> MAEYFTYSKKRKEFNNPINFQDTETRYGGIQNQVVNINQYVQRNPNFIDLDNIAELSEHSVNTERVKTGDRGMSHKEGGWPGNVDPNEAQETGRFKKRIEKDTSFPQAVKDLKEGVEKCIYQNNQIDLLEEYFEGETSEHVVENLSSKTLMLFKDEKEICKRSVSEISWHPEGPTKVAVSYAIMRFQQMPEKMPTQAYVWDLLNPNSPEIKLMSPSAVTNISYNQKIPDQIGGGCYNGLLAVWDGRKGENPIMISPVENSHYEPVTHFHWLMSKTGSECVTTSTDGKVMWWDTRKFEAGPVEKLNIIEGLGENEEIIGGTALEYNVEAGPSKFLIGTESGSILTANKKLKKPVEITTRYGLDQGRHLGPVYSINRSNQNPKYFLSVGDWSCKIWVEDLKTPIIRTKYHGSYLSDGCWSPTRSGAFFLVRRDGWMDVWDYYYRQNEIAFSHKVSDSPLTCIKINQTGGAYHNSGKLCAIGDQDGTVTILELCDSLYTMQPKEKDIINEMFEREYRKEKNLETIKKQQELAKRQVQKDMGSQKEKWEKKKLEMIETAEASFHENLAKNPVNEEEFNE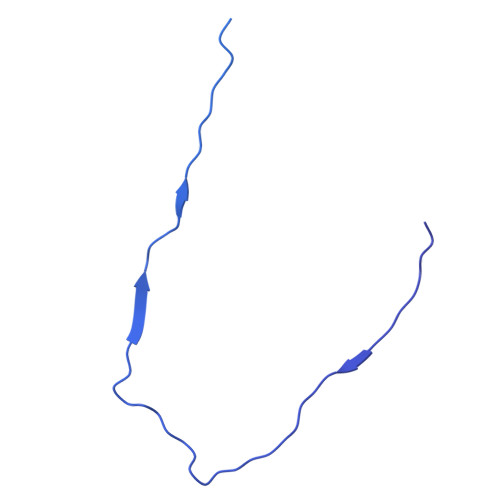LDSPSEKRKKTNQNQGREQEEQSREEQEASGNFNQQQQQQQEEEQQQEGEQQHHQNQEHQNGQGHENGQEEGEENGEEGNQQENEGQEENEQQQE>KHKEIVFGTTVGDFGDMVKEQIQAELEKKGYTVKLVEFTDYVRPNLALAEGELDINVFQHKPYLDDFKKEHNLDITEVFQVPTAPLGLYPGKLKSLEEVKDGSTVSAPNDPSNFARVLVMLDELGWIKLKDGINPLTA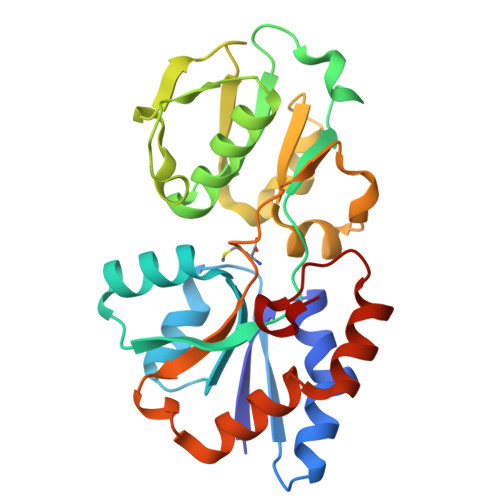SKADIAENLKNIKIVELEAAQLPRSRADVDFAVVNGNYAISSGMKLTEALFQEPSFAYVNWSAVKTADKDSQWLKDVTEAYNSDAFKAYAHKRFEGYKSPAAWNEGAAK[6x]> MEEIRNLTVK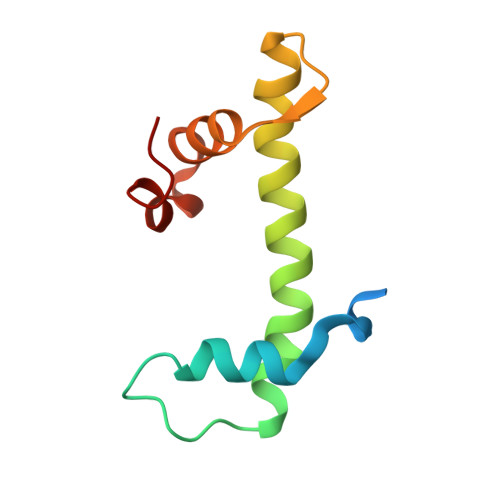DFRVQELPLARIKKIMKLDEDVKMISAEAPVLFAKAAQIFITELTLRAWIHTEDNKRRTLQRNDIAMAITKFDQFDFLIDIVPR> MSSKSEKLEKLRKLQAARNGTSIDDYEGDESDGDRIYDEIDEKEYRARKRQELLHDDFVVDDDGVGYVDRGVEEDWREVDNSSSDEDTGNLASKDSKRKKNIKREKDHQITDMLRTQHSKSTLLAHAKKSQKKSIPIDNFDDILGEFESGEVEKPNILLPSKLRENLNSSPTSEFKSSIKRVNGNDESSHDAGISKKVKIDPDSSTDKYLEIESSPLKLQSRKLRYANDVQDLLDDVENSPVVATKRQNVLQDTLLANPPSAQSLADEEDDEDSDEDIILKRRTMRSVTTTRRVNIDSRSNPSTSPFVTAPGTPIGIKGLTPSKSLQSNTDVATLAVNVKKEDVVDPETDTFQMFWLDYCEVNNTLILFGKVKLKDDNCVSAMVQINGLCRELFFLPREGKTPTDIHEEIIPLLMDKYGLDNIRAKPQKMKYSFELPDIPSESDYLKVLLPYQTPKSSRDTIPSDLSSDTFYHVFGGNSNIFESFVIQNRIMGPCWLDIKGADFNSIRNASHCAVEVSVDKPQNITPTTTKTMPNLRCLSLSIQTLMNPKENKQEIVSITLSAYRNISLDSPIPENIKPDDLCTLVRPPQSTSFPLGLAALAKQKLPGRVRLFNNEKAMLSCFCAMLKVEDPDVIIGHRLQNVYLDVLAHRMHDLNIPTFSSIGRRLRRTWPEKFGRGNSNMNHFFISDICSGRLICDIANEMGQSLTPKCQSWDLSEMYQVTCEKEHKPLDIDYQNPQYQNDVNSMTMALQENITNCMISAEVSYRIQLLTLTKQLTNLAGNAWAQTLGGTRAGRNEYILLHEFSRNGFIVPDKEGNRSRAQKQRQNEENADAPVNSKKAKYQGGLVFEPEKGLHKNYVLVMDFNSLYPSIIQEFNICFTTVDRNKEDIDELPSVPPSEVDQGVLPRLLANLVDRRREVKKVMKTETDPHKRVQCDIRQQALKLTANSMYGCLGYVNSRFYAKPLAMLVTNKGREILMNTRQLAESMNLLVVYGDTDSVMIDTGCDNYADAIKIGLGFKRLVNERYRLLEIDIDNVFKKLLLHAKKKYAALTVNLDKNGNGTTVLEVKGLDMKRREFCPLSRDVSIHVLNTILSDKDPEEALQEVYDYLEDIRIKVETNNIRIDKYKINMKLSKDPKAYPGGKNMPAVQVALRMRKAGRVVKAGSVITFVITKQDEIDNAADTPALSVAERAHALNEVMIKSNNLIPDPQYYLEKQIFAPVERLLERIDSFNVVRLSEALGLDSKKYFRREGGNNNGEDINNLQPLETTITDVERFKDTVTLELSCPSCDKRFPFGGIVSSNYYRVSYNGLQCKHCEQLFTPLQLTSQIEHSIRAHISLYYAGWLQCDDSTCGIVTRQVSVFGKRCLNDGCTGVMRYKYSDKQLYNQLLYFDSLFDCEKNKKQELKPIYLPDDLDYPKEQLTESSIKALTEQNRELMETGRSVVQKYLNDCGRRYVDMTSIFDFMLN;> MTNSVKTNGPSSSDMEYYYKSLYPFKHIFNWLNHSPKPSRDMINREFAMAFRSGAYKRYNSFNSVQDFKAQIEKANPDRFEIGAIYNKPPRERDTLLKSELKALEKELVFDIDMDDYDAFRTCCSGAQVCSKCWKFISLAMKITNTALREDFGYKDFIWVFSGRRGAHCWVSDKRARALTDVQRRNVLDYVNVIRDRNTDKRLALKRPYHPHLARSLEQLKPFFVSIMLEEQNPWEDDQHAIQTLLPALYDKQLIDSLKKYWLDNPRRSSKEKWNDIDQIATSLFKGPKQDSHIIKLRECKEDLVLMTLYPKLDVEVTKQTIHLLKAPFCIHPATGNVCVPIDESFAPEKAPKLIDLQTEMEKNNDVSLTALQPFINQFQAYVSSLLKNELGSVKREREDDDEPASLDF;> MFRQSKRRIASRKNFSSYDDIVKSELDVGNTNAANQIILSSSSSEEEKKLYARLYESKLSFYDLPPQGEITLEQFEIWAIDRLKILLEIESCLSRNKSIKEIETIIKPQFQKLLPFNTESLEDRKKDYYSHFILRLCFCRSKELREKFVRAETFLFKIRFNMLTSTDQTKFVQSLDLPLLQFISNEEKAELSHQLYQTVSASLQFQLNLNEEHQRKQYFQQEKFIKLPFENVIELVGNRLVFLKDGYAYLPQFQQLNLLSNEFASKLNQELIKTYQYLPRLNEDDRLLPILNHLSSGYTIADFNQQKANQFSENVDDEINAQSVWSEEISSNYPLCIKNLMEGLKKNHHLRYYGRQQLSLFLKGIGLSADEALKFWSEAFTNNGNMTMEKFNKEYRYSFRHNYGLEGNRINYKPWDCHTILSKPRPGRGDYHGCPFRDWSHERLSAELRSMKLTQAQIISVLDSCQKGEYTIACTKVFEMTHNSASADLEIGEQTHIAHPNLYFERSRQLQKKQQKLEKEKLFNNGNH;> MSGSIDVITHFGPDADKPEIITALENLTKLHALSVEDLYIKWEQFSNQRRQTHTDLTSKNIDEFKQFLQLQMEKRANQISSSSKVNTSTKKPVIKKSLNSSPLFGLSIPKTPTLKKRKLHGPFSLSDSKQTYNVGSEAETNEKGNSSLKLEFTPGMAEDAVGDSAPLSHAKSSDAKTPGSSTFQTPTTNTPTTSRQNVPAGEILDSLNPENIEISSGNPNVGLLSTEEPSYNQVKVEPFYDAKKYKFRTMRQNLQEASDVLDDQIESFTKIIQNHYKLSPNDFADPTIQSQSEIYAVGRIVPDSPTYDKFLNPESLSLETSRMGGVGRRVRLDLSQVNELSFFLGQIVAFKGKNANGDYFTVNSILPLPYPNSPVSTSQELQEFQANLEGSSLKVIVTCGPYFANDNFSLELLQEFIDSINNEVKPHVLIMFGPFIDITHPLIASGKLPNFPQFKTQPKTLDELFLKLFTPILKTISPHIQTVLIPSTKDAISNHAAYPQASLIRKALQLPKRNFKCMANPSSFQINEIYFGCSNVDTFKDLKEVIKGGTTSSRYRLDRVSEHILQQRRYYPIFPGSIRTRIKPKDVSTKKETNDMESKEEKVYEHISGADLDVSYLGLTEFVGGFSPDIMIIPSELQHFARVVQNVVVINPGRFIRATGNRGSYAQITVQCPDLEDGKLTLVEGEEPVYLHNVWKRARVDLIAS

The eukaryotic polymerase α (Pol α) synthesizes an RNA-DNA hybrid primer of 20–30 nucleotides. Pol α is composed of Pol1, Pol12, Primase 1 (Pri1), and Pri2. Pol1 and Pri1 contain the DNA polymerase and RNA primase activities, respectively. Here we report the cryo-EM analysis of yeast Pol α in the apo, primer initiation, primer elongation, RNA primer hand-off from Pri1 to Pol1, and DNA extension states, revealing a series of very large movements.

Upon binding template ssDNA, the Pol1-core dissociates from the platform, leading to a drastically different Pol α-primase structure to form the template-bound primer initiation state. The two-lobed elliptic apo structure now becomes three-lobed with each lobe being loosely associated with the central hinge, as evidenced by 2D class averaged images in which the position and orientation of the Pol1-core lobe, the platform lobe, and the Pri1 lobe vary. The significant conformational variability limited the achieved resolution of the EM map to 5.6 Å, insufficient to resolve the bound template ssDNA. Therefore, the ssDNA bound to human Pol α-primase is used as a placeholder for the template DNA in the yeast Pol α-primase. Transitioning from the apo state, the ssDNA template bound form of Pol1-core (i.e., state III) drops down 45 Å from the Pol12–Pol1-CTD platform and rotates 69° for binding the template DNA. Accompanying the Pol1-core movement, the Pri2-CTD rotates 92° clockwise toward the Pri1 active site for binding the template DNA, and the Pri2-NTD shifts 22 Å outwards accordingly. Therefore, both Pri1 and Pol1-core engage the template DNA, but their catalytic sites are ~49.5 Å apart. (2) In the template-bound primer initiation state, the Pri1 captures a template DNA thereby triggering a major conformational change that leads to the release of Pol1-core from the platform and the binding of the Pol1-core to the template DNA at a position that is 50 Å upstream of Pri1 (diagram 2).>[2x]SSLQIQMIGTGSAFAKKFYNNNALVKCNGFQLLIDCGVTAPRALHELGVPITGIDGILITHIHADHVGGIEEFAFRLKYKYGMTIKLFVPAAL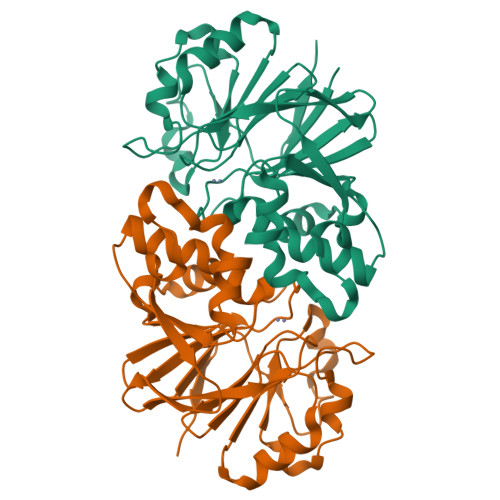VNPLWDHSLRGGLENKAEGLEQLADYFDVVALEEAVVHEIHPGLTVELVRSQHIAGKASYSLLLNNLLFYSSDARFNYAQLVELSTSGRCKYILHDCQLAEPAAVHATLNELLTLPEAVQEMIMLMHYDDEMEQFIGKSGKMSFMQQHKTYSFTEAT>GPLEDQEENTLRELRLFLRDVTKRLATDKRFNIFSKPVDIEEVSDYLEVIKEPMDLSTVITKIDKHNYLTAKDFLKDIDLICSNALEYNPDKDPGDKIIRHRACTLKDTAHAIIAAELDPEFNKLCEEIKEARIKR[2x];>[2x]CGRGKGGKGLGKG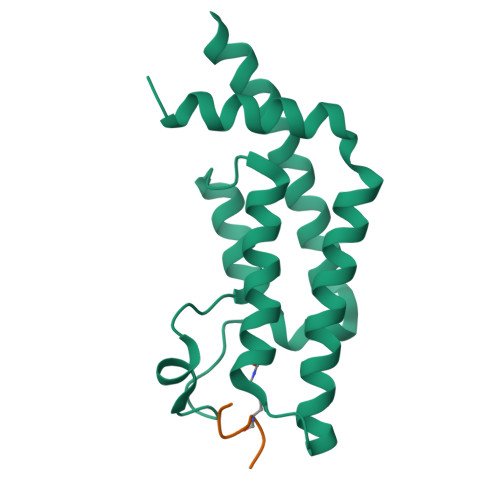GA(~{E})-3-(2-chlorophenyl)-~{N}-oxidanyl-prop-2-enamide | C9 H8 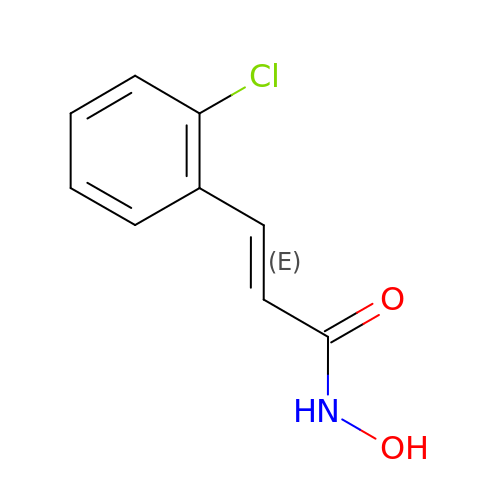Cl N O2 | HMGPSDPNANTYKH-AATRIKPKSA-N Human ubiquitin-specific protease 11 (USP11) is best known for its role in DNA damage repair by homologous recombination (HR). USP11 harbors a core protease domain as well as noncatalytic regions containing an N-terminal domain present in USPs (DUSP) and internal ubiquitin-like (UBL) domains. USP11 shares this domain architecture with paralogs USP15 and USP4, which are known as the DUSP-UBL (DU) family of USPs. We discovered USP11-specific peptides harboring consensus motifs that do not interact with either paralog USP4 or USP15, and we identified a novel binding site in the USP11 N-terminal ubiquitin-like domain.

Co-crystallization trials of USP11_DU in the presence of the FYLIR peptide yielded monoclinic crystals of space group P21 that diffracted to 1.3 Å resolution after optimization. The DUSP and UBL domains in the peptide complex structure are arranged in tandem, analogous to the structures of the rat USP11 ortholog and homologs USP4 (SGC) and USP15 (21, 22), but unlike the previous structure of human USP11_DU. Unexpectedly, the structure revealed that the peptide occupied an elongated cleft in the USP11 UBL domain, with clear electron density for peptide residues Gly-3–Arg-14 observed in both copies of the asymmetric unit. The peptide's main interacting core comprises nine residues (residues 5–13; FYKLKIRTP), with a buried interaction interface area of ∼750 Å2. Interestingly, peptide residues Glu-2–Lys-7 adopt an α-helical conformation when in complex with USP11, which is stabilized by T-shaped π–π stacking interactions of residues Phe-5 and Tyr-6. Phe-5, which can be described as the first tooth of the bidentate-like interaction, is nearly completely buried by occupying a hydrophobic pocket (referred to as major pocket). The pocket is formed predominantly by side chains of USP11 residues His-161, Trp-200, Leu-208, Ile-230, Glu-232, Pro-241, Ser-242, and Leu-245. The peptide's Ile-10 occupies a second hydrophobic pocket (USP11 Leu-245, Trp-200). Ile-10 “anchors” the peptide together with the guanidinium group of FYLIR peptide Arg-11 that forms a salt bridge with USP11 Asp-209 in what could be described as the “second tooth” of the bidentate-like interaction. The loop between strands S3 and S4 in the UBL domain (S3S4 loop, residues Asn-203–Ser-207) becomes less flexible in the peptide-bound structure due to interactions of USP11 Glu-205 with the peptide's Arg-11.

>[2x]MDREPQHEELPGLDSQWRQIENGESGRERPLRAGESWFLVEKHWYKQWEAYVQGGDQDSSTFPGCINNATLFQDEINWRLKEGLVEGEDYVLLPAAAWHYLVSWYGLEHGQPPIERKVIELPNIQKVEVYPVELLLVRHNDLGKSHTVQFSHTDSIGLVLRTARERFLVEPQEDTRLWAKNSEGSLDRLYDTHITVLDAALETGQLIIMETRKKDGTWPSAQLEHHHHHH;>[2x]AEGEFYKLKIRTPR> GAMGSGEPQSPSRRVFNPYTEFKEFSRKQIKDMEKMFKQYDAGRDGFIDLMELKLMMEKLGAPQTHLGLK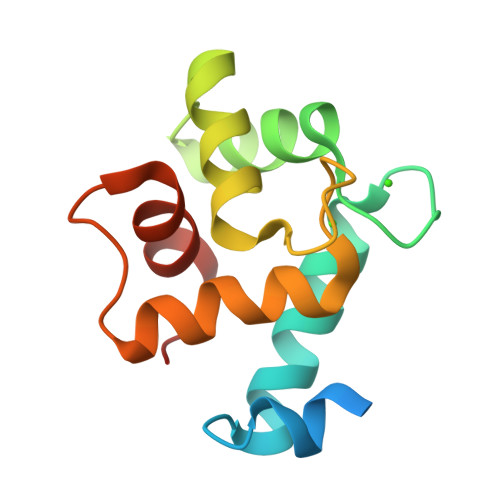NMIKEVDEDFDSKLSFREFLLIFRKAAAGELQEDSGLCVLARLSEIDVES>NDDKLYRADSRPPDEIKQSGGLMPRGQSEYFDRGTQMNINLYDHARGTQTGFVRHDDGYVSTSISLRSAHLVGQTILSGHSTYYIYVIATAPNMFNVNDVLGAYSPHPDEQEVSALGGIPYSQIYGWYRVHFGVLDEQLHRNRGYRDRYYSNLDIAPAADGYGLAGFPPEHRAWREEPWIHHAPPGCGNAPRSSMSNTCDEKTQSLGVKFLDEYQSKVKRQIFSGYQSDIDTHNRIKDEL[2x];>[10x]TPQNITDLCAEYHNTQIHTLNDKIFSYTESLAGKREMAIITFKNGATFQVEVPGSQHIDSQKKAIERMKDTLRIAYLTEAKVEKLCVWNNKTPHAIAAISMAN

One problematic target is the cholera toxin (CT), the main virulence factor of V. cholerae. CT is composed of a catalytic A-subunit (CTA) and a homopentamer of cell-binding B-subunits (CTB) that are assembled to an AB5 toxin in the periplasm. Thereafter, the multimeric toxin is secreted into the extracellular environment by the V. cholerae type II secretion system (T2SS).14−16 When produced in E. coli, we could not recover CT from the growth medium. Interestingly, assembly into holotoxins was shown to be promoted by the A-subunit, which on its own is highly unstable and prone to degradation.

To test if CT was secreted, the supernatant was directly loaded onto an IMAC column, and the elution fraction was analyzed by SDS-PAGE. Two clear bands matching the sizes of CTA and CTB were observed (last lane), confirming successful production of the toxin. CT appeared to already be almost pure after this step; nevertheless, the protein was subjected to SEC to assess the presence of CTB and remove aggregates or contaminants that may not be visible on the gel. A single sharp peak was obtained (with corresponding SDS-PAGE gel in Figure 1F), suggesting that there was little or no contamination by CTB, a major issue for expression in E. coli. For each of the independent trials of toxin production in Vmax, at least 10 times more CT was obtained in Vmax compared to E. coli (2–12 mg per L culture in Vmax vs. 0.2 mg in E. coli). By inducing expression with 0.02% l-arabinose and loading the medium on a galactose resin instead of IMAC, up to 20% higher yields were obtained. The structure was refined to R/Rfree values of 22.1/26.2% and exhibited good geometry based on the Ramachandran plot as well as small deviations from ideal bond lengths and angles. We also confirmed that the produced toxin retains its biological activity. In fact, the toxin produced in our lab elicited a stronger cAMP response in intoxicated cells than CT obtained from a commercial supplier. This difference likely relates to the greater quantity of intact holotoxin in the Vmax preparation when compared to the commercial preparation: both preparations had equivalent levels of the CTB subunit as assessed by SDS-PAGE, but the commercial preparation had a lower quantity of CTA and, thus, less functional toxin. Since expression in Vmax was performed at a lower temperature compared to E. coli (30 versus 37 °C in E. coli), we suspect that CTA may be less affected by thermal degradation in this system, leading to a more homogeneous production of the holotoxins.>[2x]MAEGERQPPPDSSEEAPPATQNFIIPKKEIHTVPDMGKWKRSQAYADYIGFILTLNEGVKGKKLTFEYRVSEAIEKLVALLNTLDRWIDETPPVDQPSRFGNKAYRTWYAKLDEEAENLVATVVPTHLAAAVPEVAVYLKESVGNSTRIDYGTGHEAAFAAFLCCLCKIGVLRVDDQIAIVFKVFNRYLEVMRKLQKTYRMEPAGSQGVWGLDDFQFLPFIWGSSQLIDHPYLEPRH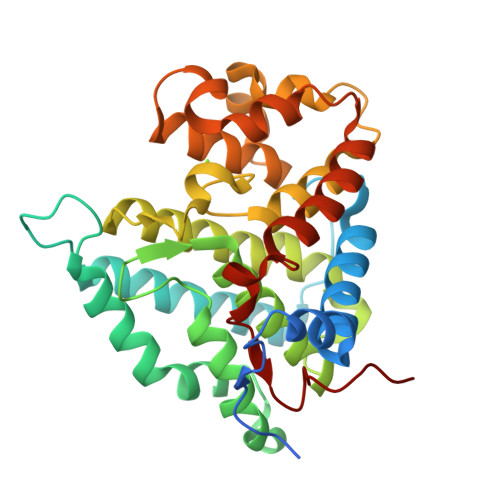FVDEKAVNENHKDYMFLECILFITEMKTGPFAEHSNQLWNISAVPSWSKVNQGLIRMYKAECLEKFPVIQHFKFGSLLPIHPVTSG>[2x]GPGSEFDPGLPSTEDVILKTEQVTKNIQELLRAAQEFKHDSFVPCSEKIHLAVTEMASLFPKR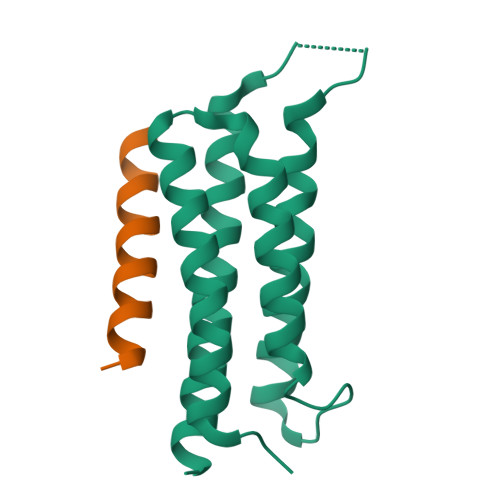PALEPVRSSLRLLNASAYRLQSECRKTVPPEPGAPVDFQLLTQQVIQCAYDIAKAAKQLVTITTREKKQ;>GPGSEFSATRELDELMASLSDFKFMAQG[2x]> SKQDQETYLETIKDFQPTELFQVLATSEDLSIDELLRDSLESYSQDRDRFLQEFINLLLCCCGAIARLEVHDVHSNESSNETVGELQLLFQRQKVHEFHLLISKDSKKKSKYPPLYANFVEFMFRLMDVANDLQLLYVESDEDESEIGTGPLIIDLLTWLSPLSVCKIRSLRYIATLTLYLFQDFLTDHVVDLDKNYLSKLSKQLSVENKKKRPNGKTVEKLESTIAEIQSSKMVTQGIIDNIIKLCFVHRFKDVDETIRCESMVHLASWTKSFPEYFLKVTFLKYFGWLLSDSSVTVRLQVLKILPQLISQHHNRAVDNSAVRQFFERFKERILEIALKDSNLEVRLSAVQVLVEVASLGYLEDTEILSISSLIFEDNEIKVSSLGKNSRYLASVAKFFACITEEKFQEFTNNRVLPKELFDVKGSSAVRIGIFMNLLNESLTEYLQKVPQIGSEKRIHILFQAAEFLYPYFGSLIKDICKVLTFEGEFTHESLETPTYTGDNNNEENNDENNRSNLLLPTDSNNIILYVTTLHGLAYGGTHMRGQPKFKVAEAVLPHLDQLIKRLPIESSNVLASILGVFNLFAFEDWIHTGYEKDIRKILEKIIKAFNESTLTSGAQDLKYKSFSETVSQVRKLGFNELDELWLNHIS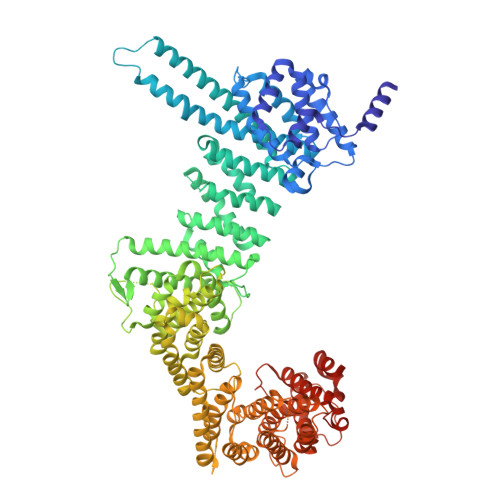QLKIHLGKFLEEKLHPDVQDTENDENMNTLYGVFLNKLALLGKVYPIEFQENLLSLFLNRFVQRLPQIGVHCQLETIQEIHLKLLALLTTWQLQKWVDILEKSSENDSPSPVSEFSLRTVSSIVKSFKVIFDALSSDTNDNDGTLGDFLLKWSTSNSFIDIIISLKVFELGVAESEKSWRHALRENFVPYVTDSANQVLLKVFLYLESLFANESSEHLDRNPQEDVNLNDIKYDGFGDGCEKELLLFTIKLKGLMKLGLLDEALFSRIALNKEKLGPLYAKVIEDTIFDQDKKGRVPHHHHHH>MSKKHTGYVGLKNQGATCYMNSLLQTLFFTNQLRKAVYMMPTEGDDSSKSVPLALQRVFYELQHSDKPVGTKKLTKSFGWETLDSFMQHDVQELCRVLLDNVENKMKGTCVEGTIPKLFRGKMVSYIQCKEVDYRSDRREDYYDIQLSIKGKKNIFESFVDYVAVEQLDGDNKYDAGEHGLQEAEKGVKFLTLPPVLHLQLMRFMYDPQTDQNIKINDRFEFPEQLPLDEFLQKTDPKDPANYILHAVLVHSGDNHGGHYVVYLNPKGDGKWCKFDDDVVSRCTKEEAIEHNYGG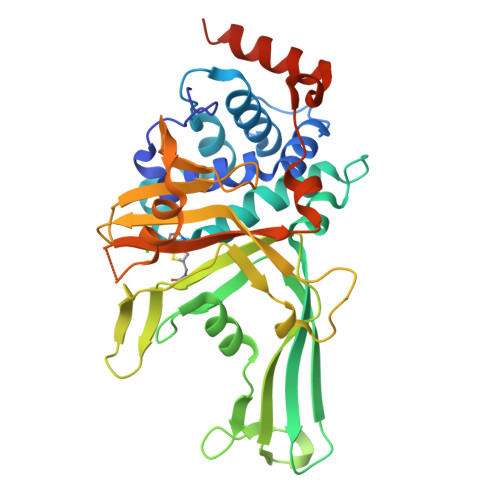HDDDLSVRHCTNAYMLVYIRESKLSEVLQAVTDHDIPQQLVERLQEEKRIEAQKRKERQEHHHHHH[2x]One especially common junction element is the kink-turn (k-turn). k-turns are elements in double-stranded RNA that introduce a tight kink into the helical axis, with an included angle close to 50°. A standard k-turn comprises a three-nucleotide bulge followed by successive G•A and A•G trans G(sugar edge)•A(Hoogsteen edge) basepairs. k-turns are commonly-occurring motifs that introduce sharp kinks into duplex RNA, thereby facilitating tertiary contacts. Both the folding and conformation of k-turns are determined by their local sequence. k-turns fall into two conformational classes, called N3 and N1, that differ in the pattern of hydrogen bonding in the core. We show here that this is determined by the basepair adjacent to the critical G•A pairs.

We therefore decided to extend the study with a systematic structural analysis of HmKt-7 as a function of the 3b,3n sequence. This was performed in the constant environment of the SAM-I riboswitch, modified by replacing its natural k-turn by HmKt-7 with different 3b,3n sequences. In this way we could observe the effect of changing the 3b,3n sequence alone in an otherwise completely unchanged RNA molecule. Additionally, we hoped we might expand the range of 3b,3n sequences beyond the eight found in the natural k-turns to date. Six are completely new, i.e. 3b,3n = C•A, C–G, C•U, G•G, U–A and U•C, five of which adopt the N1 conformation. We note the majority (6/8) of the 3b = pyrimidine k-turns form N1 structures. Altogether seven of the new structures are in the N1 conformation, and clearly simply changing the 3b,3n sequence alone is sufficient to induce the structure of Kt-7 to change within the riboswitch environment. Evidently the 3b,3n sequence is the major determinant of the k-turn conformation.

> GGCUUAUCAAGAGAGGGUGAGCGACUGGCGCGAAGACCCCCGGCAACCAGAAAUGGUGCCAAUUCCUGCAGCGGAAACGUUGAAAGAUGAGCCG Here, we demonstrated that SatS, which we revealed is required for M. tuberculosis growth in macrophages, functions in the export of SapM and an additional subset of the proteins exported by the SecA2 pathway. We further identified properties of SatS that indicate a function as a protein export chaperone that protects its substrates from inappropriate interactions in the cytoplasm and additionally assists in their export. SatS is a highly acidic (pI 3.83), cytoplasmic protein with a role promoting export of a subset of the proteins exported by the SecA2 pathway. Finally, we determined the structure of the C-domain of SatS (SatSC), which reveals a new fold lacking similarities to any solved chaperone structures, yet contains surface hydrophobic grooves resembling those of the SecB chaperone.

Subsequently, constructs expressing SatSC or SatSN in E. coli were used to purify the individual domains to homogeneity for crystallization trials. Only SatSC yielded diffraction quality crystals diffracting to 1.4 Å resolution. SatSC displays α/β secondary structure comprised of a mostly parallel, four stranded β-sheet core, flanked by seven α-helices. The structure revealed a new fold sharing no similarities with any previously solved protein structure in the PDB based on DELTA-BLAST and VAST similarity searches. Although the overall polypeptide fold was not similar to known proteins, the surface of SatSC had pronounced electronegative charge potential that is comparable to many export chaperones, including SecB. Furthermore, the SatSC structure featured two surface localized hydrophobic grooves, mapped by the Kyte-Doolittle hydrophobicity scale. These grooves bore similarity to the hydrophobic grooves on SecB that serve as primary and secondary client binding sites to regions of unfolded preproteins. The proximity of the smaller hydrophobic groove in SatSC (Site 2) to the larger groove in SatSC (Site 1) as well as their amino acid composition (aromatic and bulky side chains) resembled the arrangement and composition of the client binding sites of SecB. The larger of the two hydrophobic grooves in SatSC (Site 1) was comparable in size to the ~60 Å long, main binding site in SecB. In fact, when we tested SatSC for chaperone activity in the in vitro anti-aggregation assay, SatSC alone was sufficient to ablate preSapM-HIS aggregation comparable to full length SatS.

> SHMVVLGGDRDFWLQVGIDPIQIMTGTATFYTLRCYLDDRPIFLGRNGRISVFGSERALARYLADEHDHDLSDLSTYDDIRTAATDGSLAVAVTDDNVYVLSGLVDDFADGPDAVDREQLDLAVELLRDIGDYSEDSAVDKALETTRPLGQLVAYVLDPHSVGKPTAPYAAAVREWEKLERFVESRLRRE1-{2-deoxy-5-O-[(S)-hydroxy{[(S)-hydroxy(phosphonooxy)phosphoryl]oxy}phosphoryl]-beta-L-erythro-pentofuranosyl}-5-methylpyrimidine-2,4(1H,3H)-dione | C10 H17 N2 O14 P3 | 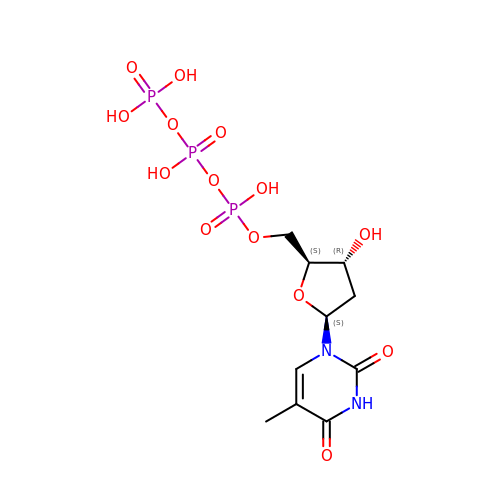NHVNXKFIZYSCEB-CSMHCCOUSA-N> VDCSEYPKPACTIEYRPLCGSDNKTYGNKCNFCNAVVESNGTLTLS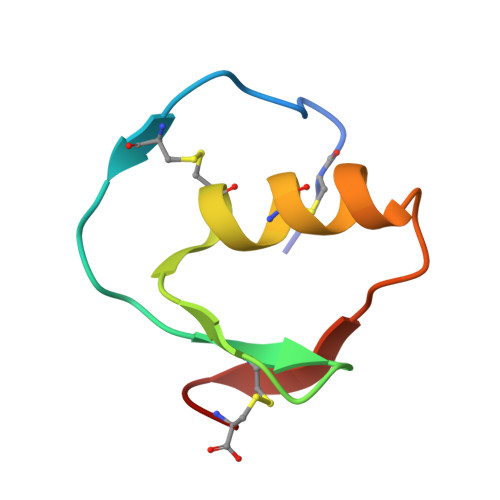HFGKC>[2x]MTRPEQPRPESADLPAPTLEVIPLGGMGEIGKNITVFRYGDEIVVVDGGLAFPKAHQMGIDLIVPRIDYLLEHQDKIKGWILTHGHEDHIGGLPYIFARLPRVPVYGLPLTLALVREKLSEFGLQDVDLREVTYGDEVRFGQSFVAEFFCMTHSIPDNAGYILKTPVGDVLHTGDFKIDPDVGTGAGIVSDLERVEQAGKDGVLLLISDSTNAERPGHTPSEAEIARNLEEIIKGCRGRVFLTTFASQVYRIQNILDLAHRQGRRVVMEGRSMIKYAQAAQATGHMNPPEPFLTSEEVGELQDQQVLFVCTGSQGQPMAVLGRLAFGTHAKIALRRGDTVILSSNPIPGNEDAVNLIVNRLYEIGVDVVYPPTYRVHASGHASQEELATILNLTRPKFFLPWHGEPRHQINHAKLAQTLPRPPKRTLIAKNGDIVNLGPDEFRVSGTVAAGAVYVDGLGVGDVNDDVLLDRVNLSQEGLLILTAV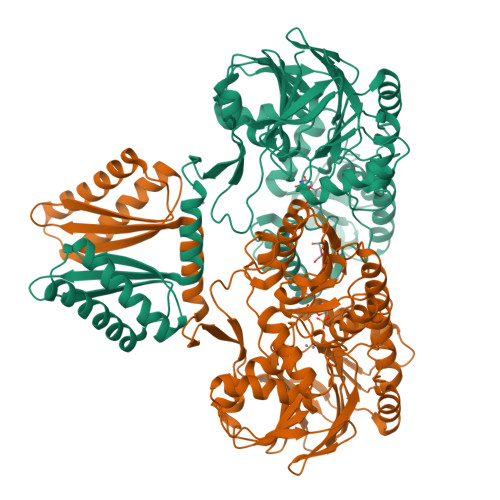LHPTPHVEVVARGFARPNRDLELQIRRVALEAVEQGLREKKRLEDVRDDMYGAVRRFTRKATGRNPVLIPMIVD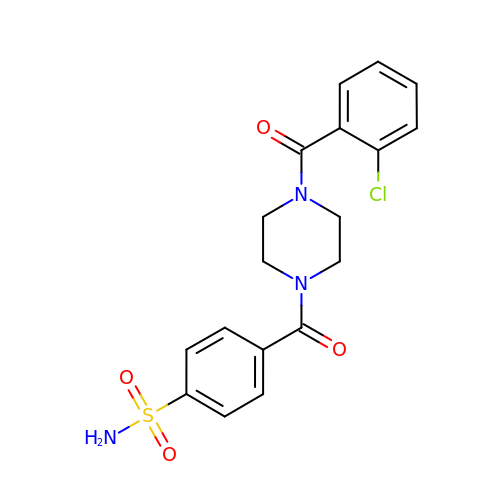4-[4-(2-chlorophenyl)carbonylpiperazin-1-yl]carbonylbenzenesulfonamide | C18 H18 Cl N3 O4 S | ZWAGEDFCAJXKDS-UHFFFAOYSA-N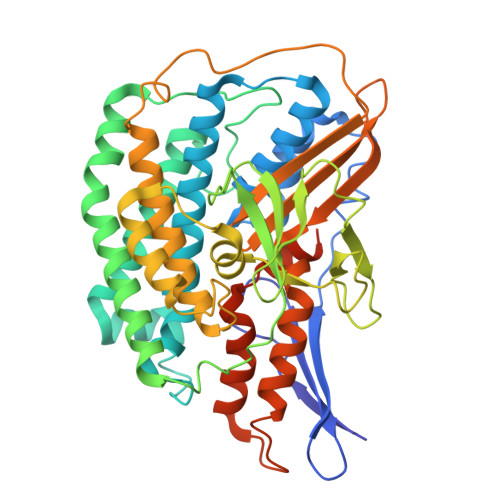> MTEVFKLEINPVTRIEGHGKITVMLDESGHVRETRFHVTQYRGFEVFTHGRDFREMPVITPRICGICPVSHHLASAKACDEILGVTITPAAHKLRELMHMGQIVQSHALSFFHLSSPDILWGFDAPVKIRNVAGLVDRYPELAKKGIMLRKFGQEIIKTLGGKKIHPWHSIPGGVNRSLTPQERDAIAAQLPEMKSIAMEAIKLIKDYLQEGGEELKEFATLDTAYMGLVRDGYLELYDGEVRIKAPRGRILDQFDPKDYLDHIGEHVEPWSYLKFPFYKALGFPHGSYRVGPLARLNAADAVSTPEASKEFALYKEMGEDGIVPYTLYYHYARLIEALYGLERIEQLLADPDITSSDLRVTSKEINPEGIGVIEAPRGTLIHHYQVNESGVITKVNLIVATGHNNFAMNKGVEMVAKKYITGTNVPEGVFNRLEHVIRAYDPCLSCSTHAVGKMPLKLELVGPTGEILKEVTRD> MTQRKRAARWVGIPCAILFLTVPFISATASTPGPASTAEPKVDAIVIDTAAVFGKLEQPGVVFYHEKHTTALEKMAKDCTSCHVETEGKLSFKFARTVDPTSKNAMAEQYHANCMACHEKVVGSYPTAPQAAECKRCHVGPGVEGATVTPKPSLDLNLHGRHVVAEAKRLQVKEDESCKACHHTYDEAQKKLVYAKGEEGSCVYCHKQEPLPSPVQQDRVVPSTRDASHESCVNCHLSTRKAQTESGPVLCVGCHTAEAQAAWKKTAETPRLFRGQPDATLLVAGAATANGTVDVNWAAAGPGPVAFDHKAHEGFVGNCVTCHHPTQTGGSLAACGVACHTTTGSKDGNFVTTAQSAHQLGVTTSCVGCHTTQANARKECAGCHAPMQKTALSQNSCIQCHEAGFPTSGTQTLGKEEREATAAKILAAKDEKP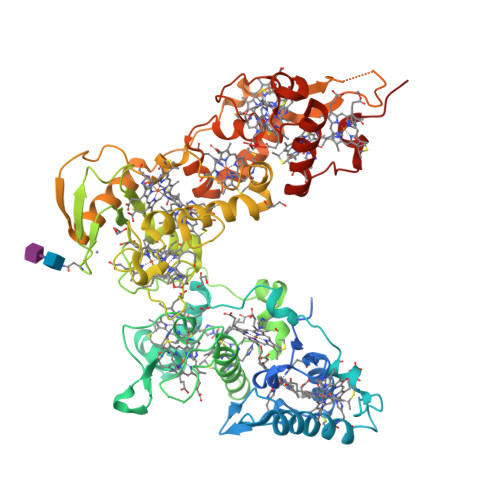KTVPLENVPEKLTLNYMDEKGDEWQAAEFPHRKIYQKLVEEAAKSPMANHFHGDALTMCSGCHHNAKPSLNPPKCASCHSKPFQERTANQPGLKGAFHNQCIGCHQEMQVNPKATDCQGCHKPKNSA> MKKSIRRSGGKSK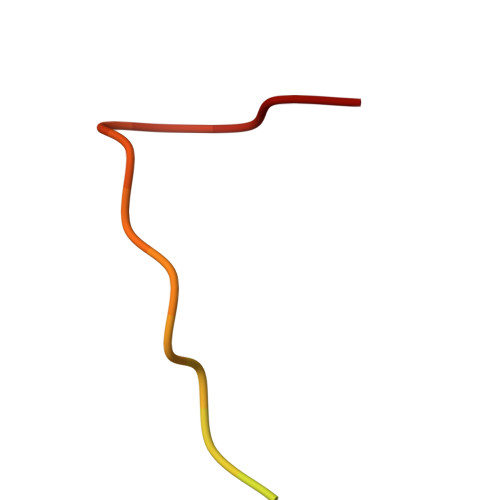GARLWYVGGTQY>[2x]AVINTFDGVADYLIRYKRLPDNYITKSQASALGWVASKGNLAEVAPGKSIG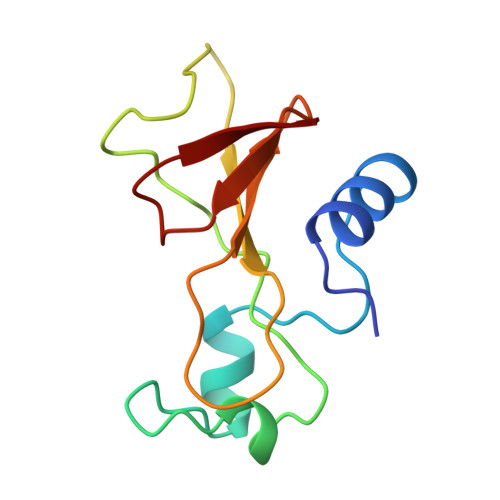GDVFSNREGRLPSASGRTWREADINYVSGFRNADRLVYSSDWLIYKTTDNYATFTRIR>[30x]MATPWSGYLDDVSAKFDTGVDNLQTQVTEALDKLAAKPSDPALLAAYQSKLSEYNLYRNAQSNTVKVFKDIDAAIIQNFR

The injectisome is a specialized bacterial organelle that utilizes a type III secretion system (T3SS) to translocate effector proteins from the bacterial cytosol directly into a eukaryotic host. Composed of >20 different proteins, the injectisome forms a syringe shaped nanomachine that spans both bacterial membranes and that of the infected host. The major structural unit of the injectisome is the basal body, composed of three highly oligomerized concentric rings spanning the bacterial inner membrane (IM) (PrgH and PrgK in the Salmonella enterica serovar Typhimurium SPI-1 T3SS)3–6 and outer membrane (OM)7 (InvG, a member of the secretin family of OM pores also found in the type II secretion system, type IV pili system, as well as the phage assembly system). To address this and further elucidate the structural basis for injectisome assembly and function, including that of the central needle component, we have conducted here a cryo-EM analysis of the assembled native needle complex resulting in 3D reconstructions of the IM and OM rings at resolutions permitting atomic model building (3.6 Å and 3.9 Å, respectively) and the 3D reconstruction of an isolated helical needle filament at 3.3 Å resolution.

Completing assembly, the helical needle filament—composed of early substrates PrgJ (the rod) and PrgI (the needle)—is secreted in a type III secretion (T3S) dependent manner and polymerizes on the periplasmic face of the export apparatus, extending into the cellular milieu. To further study the atomic details of the needle therefore, we isolated native filaments from assembled needle complexes and subjected them to cryo-EM analysis resulting in a reconstruction with helical averaging to 3.3 Å resolution with excellent density for side chains throughout allowing us to build a de novo model of PrgI lacking only the first two N-terminal residues. The PrgI monomer adopts a helix-turn-helix motif that polymerizes via an extensive network of interactions along both helices with surrounding subunits. The structure supports the solid-state NMR model of PrgI presented by Loquet et al. (Cα RMSD 1.5 Å over 78 residues), which was fundamentally different from prior low resolution cryo-EM derived models; however, some notable differences in the monomeric structure and helical packing, as well as the definition of the majority of side chain positions extend our understanding of the intra-subunit interactions and the internal channel passaged by effectors. The kinked loop in the N-terminal helix (residues 20–23) is more extended and forms a tighter interface with the N-terminus of monomer i + 6 while the C-terminal Arg80 has its side chain and carboxylate flipped, altering the interactions with monomers i −1, i –5, and i – 6.>MKMLEQLEKKLGYTFKDKSLLEKALTHVSYSKKEHYETLEFLGDALVNFFIVDLLVQYSPNKREGFLSPLKAYLISEEFFNLLAQKLELHKFIRIKRGKINETIIGDVFEALWAAVYIDSGRDANFTRELFYKL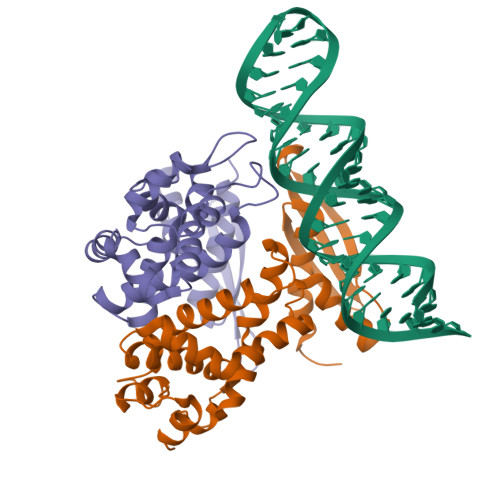FKEDILSAIKEGRVKKDYKTILQEITQKRWKERPEYRLISVEGPHHKKKFIVEAKIKEYRTLGEGKSKKEAEQRAAEELIKLLEESE[2x]> XTDAVLELPAATFDLPLSL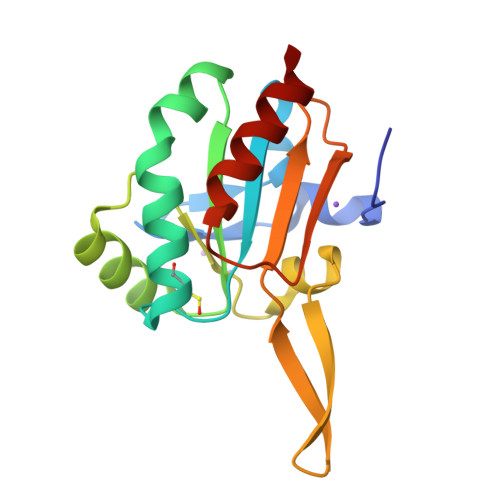SGGTQTTLRAHAGHWLVIYFYPKDSTPGCTTEGLDFNALLPEFDKAGAKILGVSRDSVKSHDNFCAKQGFAFPLVSDGDEALCRAFDVIKEKNMYGKQVLGIERSTFLLSPEGQVVQAWRKVKVAGHADAVLAALKAHAKQ>GPGMATEEMKKLATVMAIGTANPPNCYYQADFPD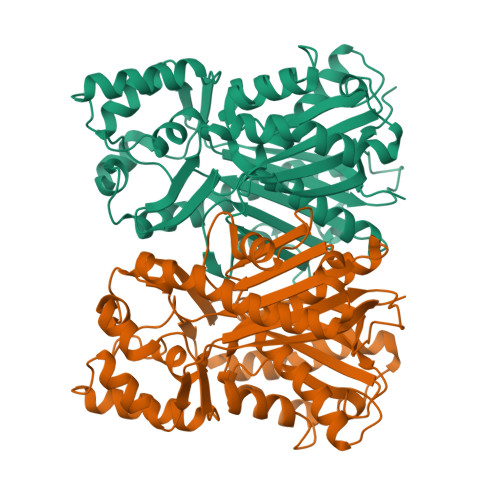FYFRVTNSDHLINLKQKFKRLCENSRIEKRYLHVTEEILKENPNIAAYEATSLNVRHKMQVKGVAELGKEAALKAIKEWGQPKSKITHLIVCCLAGVDMPGADYQLTKLLDLDPSVKRFMFYHLGCYAGGTVLRLAKDIAENNKGARVLIVCSEMTTTCFRGPSETHLDSMIGQAILGDGAAAVIVGADPDLTVERPIFELVSTAQTIVPESHGAIEGHLLESGLSFHLYKTVPTLISNNIKTCLSDAFTPLNISDWNSLFWIAHPGGPAILDQVTAKVGLEKEKLKVTRQVLKDYGNMSSATVFFIMDEMRKKSLENGQATTGEGLEWGVLFGFGPGITVETVVLRSVPVIS[2x]> MGSMIVFRYLSREVLVTMSAVSAVLLVIIMSGRFIKYLA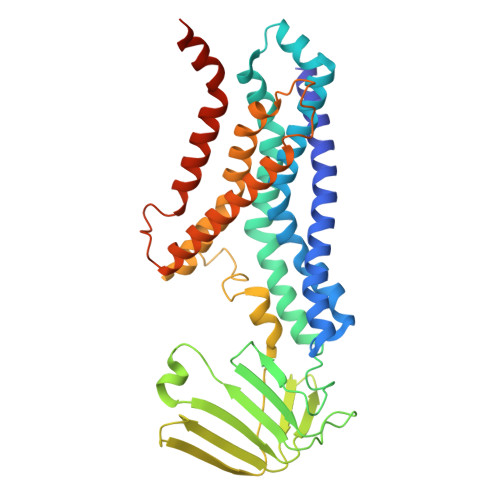QAAQGLLDPGSLFLIMAFRIPGFLQLILPLGLFLGILLAYGRLYLESEMTVLSATGMSQKRLLGYTMAPALLVAILVAWLSLFLAPQGINQFALLLNKQDTLTEFDTLVPGRFQAMRDGTRVTYTEELSKDRGELAGIFISQKDLNSSNQERGISILVAEKGTQNIQADGSRYLILHNGYRYDGNPGQANYRAIQYDTYGVMLPKPEASSEVSERDAVPTADLFGSDNPRYQAELQWRLSTPLLVFVVTLLAVPLSRVNPRQGRFLKLLPAILLYMGYLALLIAVRGQLDKGKIPMAIGLWWVHGLFLAIGLLLFYWEPLRLKLASSRAGREVAHG> MALK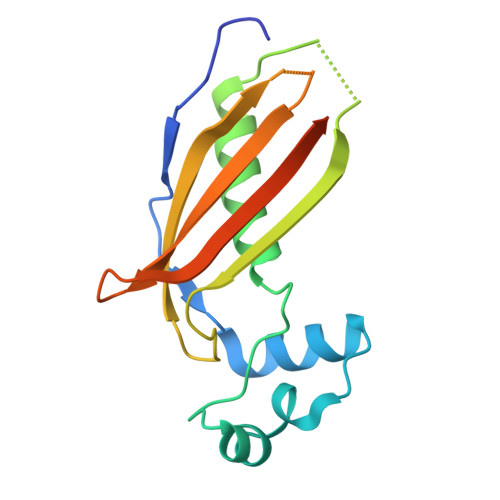TDIRGMIWRYPDYFIVGREQCREFARAVKCDHPAFFSEEAAADLGYDALVAPLTFVTILAKYVQLDFFRHVDVGMETMQIVQVDQRFVFHKPVLAGDKLWARMDIHSVDERFGADIVVTRNLCTNDDGELVMEAYTTLMGQQGDGSARLKWDKE>[6x]AKLVFF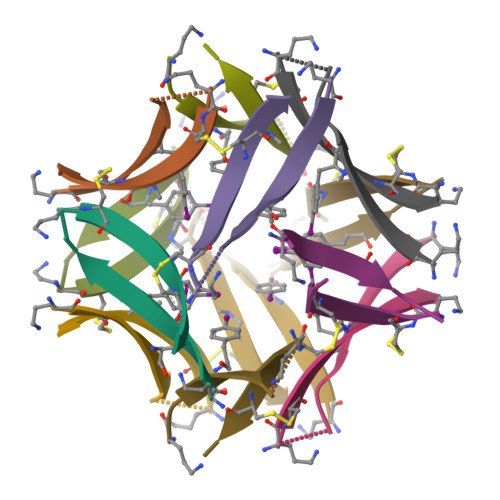AEACIIGCMV>QGMTKVAIVTASDSGIGKACALLLAQNGFDIGITWHSDERGAQETAKKAAQFGVRAETIHLDLSQLPEGAQAIEHLIQRLGRVDVLVNNAGAMTKSAFID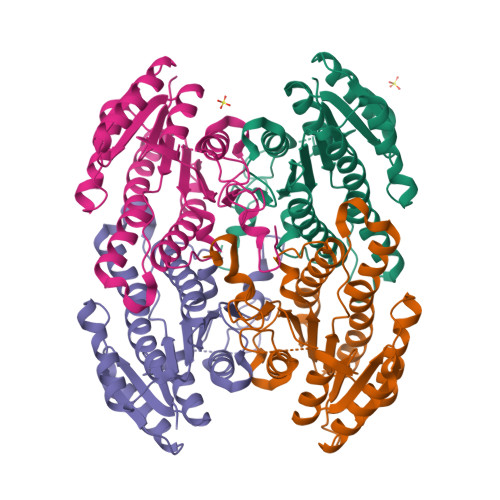MPFTQWRQIFTVDVDGAFLCAQIAARHMIKQGEGGRIINITSVHEHTPLPQASAYTAAKHALGGLTKSMALELIEHHILVNAVAPGAIATPMNDMDDSDIEPGSEPSIPIARPGSTHEIASLVAWLCSEGASYTTGQSLIVDGGFMLANPQFNAK[8x]AKAP-Lbc (also known as AKAP13) is a member of the A-kinase-anchoring proteins. AKAP-Lbc exists as at least three splice variants, however, all contain a conserved RhoGEF (Rho GTPase guanine-nucleotide-exchange factor) domain. RhoGEF domains decrease the affinity of a Rho GTPase for GDP so that GTP, present in higher concentrations in the cell, can bind. RhoGEF domains are composed of a DH (Dbl-homologous) domain followed by a PH (pleckstrin homology) domain.

To investigate whether for our constructs the AKAP-Lbc PH domain contributes to catalysis of nucleotide exchange on RhoA we cloned an expression construct containing just the DH domain (residues 1976–2211, terminating at the end of αI) for comparison with the combined DH–PH domain. To analyse conformational changes in the DH domain on binding we crystallized the DH domain alone in the absence of RhoA, revealing a significant movement of the GEF switch region, which adopts an α-helical conformation with Trp1980 itself binding in a different pocket on the first DH domain α-helix. This we refer to as the inactive conformation, in which the position occupied by Trp1980 in the active conformation is now occupied by Ile1984 and Ile1983. In this inactive conformation, the critical Glu2001 can no longer bind to RhoA. We cannot rule out that the inactive α-helical conformation is induced by the N-terminal protein tag which is at the start of this α-helix. However, we note that the region around Trp1980 is weakly predicted to be α-helical by the PsiPred server, suggesting that a conformational exchange in and out of an α-helix induced by the absence or presence of RhoA is a realistic model. In contrast with AKAP-Lbc, in the structure of p115-RhoGEF in the absence of RhoA, the GEF switch maintains an active conformation.

>[2x]ENLYFQSMEAESWSRIIDSKFLKQQKKDVVKRQEVIYELMQTEFHHVRTLKIMSGVYSQGMMADLLFEQQMVEKLFPCLDELISIHSQFFQRILERKKESLVDKSEKNFLIKRIGDVLVNQFSGENAERLKKTYGKFCGQHNQSVNYFKDLYAKDKRFQAFVKKKMSSSVVRRLGIPECILLVTQRITKYPVLFQRILQCTKDNEVEQEDLAQSLSLVKDVIGAVDSKVASYEKKVRLNEIYTK> SMLEAKFEEASLFKRIIDGFKDCVQLVNFQCKEDGIIAQAVDDSRVLLVSLEIGVEAFQEYRCDHPVTLGMDLTSLSKILRCGNNTDTLTLIADNTPDSIILLFEDTKKDRIAEYSLKLMDIDADFLKIEELQYDSTLSLPSSEFSKIVRDLSQLSDSINIMITKETIKFVADGDIGSGSVIIKPFVD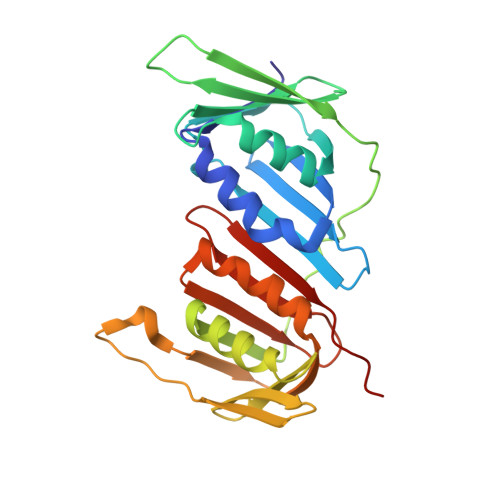MEHPETSIKLEMDQPVDLTFGAKYLLDIIKGSSLSDRVGIRLSSEAPALFQFDLKSGFLQFFLAPKFNDEE>MSQSGEDLHSPTYLSWRKLQLSRAKLKASSWTSALLSGFAMVAMVEVQLDHDTNVPPGMLIAFAICTTLLVAVHMLALMISTCILPNIETVSNLHSISLVHESPHERLHWYIETAWAFSTLLGLILFLLEIAILCWVKFYDLSPPAAWSATVVLIPVMIIFMAFAIHFYRSLVSHKYEVTVSGIRELEMLKEQMEQDHLEHHNNIRNNGEGEEF[3x]

Orai was identified as the protein that forms the channel’s pore and STIM was identified as its regulator. The channel is activated by the depletion of Ca2+ from the endoplasmic reticulum (ER), and as such it was characterized as the calcium release-activated calcium (CRAC) channel responsible for store-operated calcium entry (SOCE) before the molecular components were known. The channel is formed from an assembly of six Orai subunits that surround a single ion pore, which is perpendicular to the plasma membrane in a cellular setting. Each Orai subunit contains four transmembrane helices (M1-M4) and a cytosolic M4-ext helix.

We also obtained crystals of K163W Oraicryst in a P42212 crystal form that diffracted X-rays to 4.35 Å resolution, which assisted with model building and was indistinguishable from the I41 structures of WT and K163W Oraicryst. The K163W mutation corresponds to R91W in human Orai1, which is a loss of function mutation that causes a severe combined immune deficiency-like disorder. The structures of WT and K163W Oraicryst reveal an ‘unlatched-closed’ conformation of the channel that resembles a hybrid of the quiescent and open conformations: the ion pores are closed as in the quiescent conformation but the M4/M4-ext regions have conformations like those observed in the H206A Oraicryst structure. The conformation of the M1-M4a portion of the channel, however, is like the quiescent conformation, and as such, the pores of WT and K163W Oraicryst are closed and indistinguishable from the pore in the structure of the quiescent conformation. The density is positioned roughly in the center of the basic region in the structure of WT Oraicryst and located in the lower portion of it in the structures of the K163W mutant, which removes the top ring of basic residues from the pore. The K163W mutation has no other apparent effect, and this is analogous to observations from structures of the quiescent conformation with and without the K163W mutation. Congruently, we observe that the corresponding K163W mutant of Drosophila Orai can adopt an unlatched conformation with a closed pore. Our observation that the unlatching of M4b from M3 does not necessarily open the pore is consistent with studies indicating that STIM1 can bind to loss-of-function mutants of human Orai1 that have constitutively closed pores, such as the pore-lining R91W mutant.> GGUGACUAGGGUUCCGGCGAAAGCCGGUCCGAGAGUUACCGACCGCCGAAAGGCG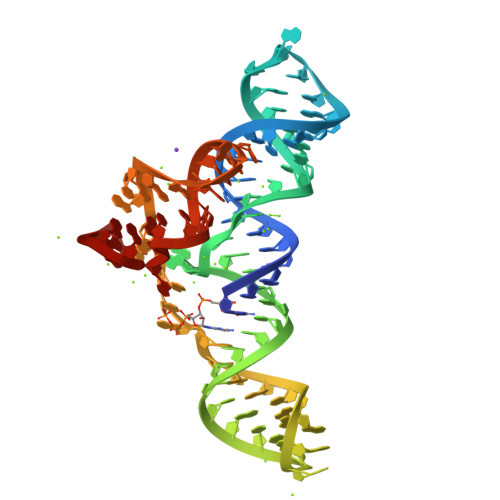GUUACACGGCGGGAAAAAAGCCCGGGAGGA Enzymes belonging to the purine salvage pathway are potential targets for novel drugs against H. pylori, as recent studies have shown that this bacterium is unable to synthesise purine nucleotides de novo. Furthermore, its growth was notably hampered in a medium abundant in nutrients. These results strongly suggest that AdSS is critical for the survival of H. pylori. Using a broad set of microbiological, physicochemical (UV absorption, LC-MS, X-ray analysis) and in silico experiments, we were able to prove that PLP inhibits adenylosuccinate synthetase (AdSS) from H. pylori by the competition with GTP (IC50eq ∼30 nM). The core of the enzyme comprises a β-sheet composed of 9 β-strands (8 mutually parallel and one anti-parallel), flanked by more than 10 α-helices of various length.

C-His tag AdSS was complexed with two out of its three substrates (IMP and Asp) and with PLP, in the presence of Mg2+. GTP was omitted, as according to the studies described above it competes with PLP, hence we expect to find PLP in the GTP-binding site. Our findings reveal that the AdSS-ligand complex crystallises in the I 1 2 1 space group, with a monoclinic unit cell of dimensions 69.9 Å, 62.1 Å, 119.3 Å, 90.0°, 98.9°, 90.0°. The asymmetric unit contains one monomer of the protein (thus half of the functionally capable enzyme). Ligands bound in the active site are IMP and PLP, even though before crystallisation AdSS was preincubated with four potential ligands: IMP, Asp, PLP and Mg2+. However, the long side chain of Arg135 from the neighbouring subunit extends towards the active site of the paired monomer and participates in the ligand binding, namely in binding of IMP, thus indicating the necessity of a dimeric architecture for the formation of the catalytically active AdSS. Phosphate group of PLP is clearly visible in the electron density. It is located in the position of β phosphate group of GTP (GDP), and it maintains the hydrogen bond network of this phosphate group, namely forms hydrogen bonds with backbone atoms of Lys15 and Gly14, and with Nζ of Lys15. The aromatic ring of PLP is bound covalently to the side chain atom Nζ of Lys322 utilising for this purpose the aldehyde group of PLP. The distance between C4A atom of PLP and Nζ atom of the Lys322 is 1.26 Å, thus confirming formation of the covalent bond formation.

> MADVVVGIQWGDEGKGKIVDRIAKDYDFVVRYQGGHNAGHTIVHKGVKHSLHLMPSGVLYPKCKNIISSAVVVSVKDLCEEISAFEDLENRLFVSDRAHVILPYHAKKDAFKEKSQNIGTTKKGIGPCYEDKMARSGIRMGDLLDDKILEEKLNAHFKAIEPFKKAYDLGENYEKDLMGYFKTYAPKICPFIKDTTSMLIEANQKGEKILLEGAQGTLLDIDLGTYPFVTSSNTTSASACVSTGLNPKAINEVIGITKAYSTRVGNGPFPSEDTTPMGDHLRTKGAEFGTTTKRPRRCGWLDLVALKYACALNGCTQLALMKLDVLDGIDAIKVCVAYERKGERLEIFPSDLKDCVPIYQTFKGWEKSVGVRKLDDLEPNVREYIRFIEKEVGVKIRLISTSPEREDTIFL>KEAETQQKLANVVILATGGTIAGAGASAANSATYQAAKLGVDKLIAGVPELADIANVRGEQVMQIASESISNDDLLKLGKRVAELAESKDVDGIVITHGTDTLEETAFFLNLVEKTDKPIVVVGSMRPGTAMSADGMLNLYNAV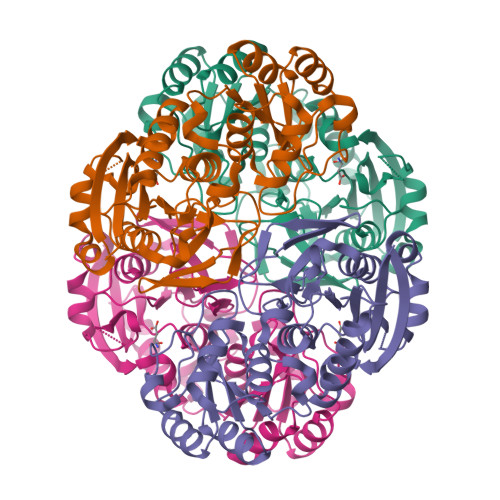AVASDKQSRGKGVLVTMNDEIQSGRDVSKAVNIKTEAFKSAWGPMGMVVEGKSYWFRLPAKRHTVNSEFDIKQISSLPQVDIAYGYGNVTDTAYKALAQNGAKALIHAGTGNGSVSSRVVPALQELRKNGVQIIRSSHVNQGGFVLRNAEQPDDKNDWVVAHDLNPQKARILAMVAMTKTQDSKELQRIFWEY[4x]> KQVSWKLVTEYAMETKCDDVLLLLGMYLEFQYSFEMCLKCIKKEQPSHYKYHEKHYANAAIFADSKNQKTICQQAVDTVLAKKRVDSLQLTREQMLTNRFNDLLDRMDIMFGSTGSADIEEWMAGVAWLHCLLPKMDSVVYDFLKCMVYNIPKKRYWLFKGPIDSGKTTLAAALLELCGGKALNVNLPLDRLNFELGVAIDQFLVVFEDVKGTGGESRDLPSGQGINNLDNLR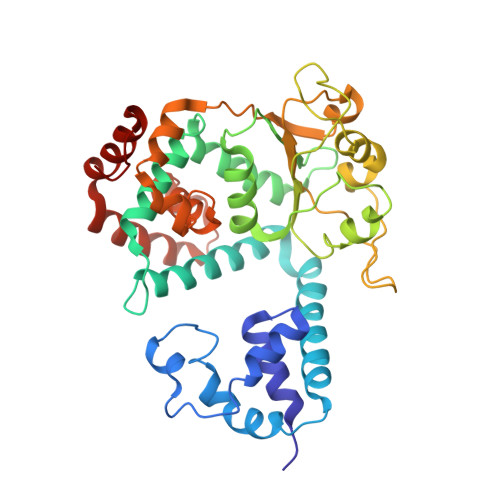DYLDGSVKVNLEKKHLNKRTQIFPPGIVTMNEYSVPKTLQARFVKQIDFRPKDYLKHCLERSEFLLEKRIIQSGIALLLMLIWYRPVAEFAQSIQSRIVEWKERLDKEFSLSVYQKMKFNVAMGIGVLD>MIGYQIYVRSFRDGNLDGVGDFRGLKNAVSYLKELGIDFVWLMPVFSSISFHGYDVVDFYSFKAEYGSEREFKEMIEAFHDSGIKVVLDLPIHHTGFLHTWFQKALKGDPHYRDYYVWANKETDLDERREWDGEKIWHPLEDGRFYRGLFGPFSPDLNYDNPQVFDEMKRLVLHLLDMGVDGFRFDAAKHMRDTIEQNVRFWKYFLSDLKGIFLAEIWAEARMVDEHGRIFGYMLNFDTSHCIKEAVWKENTRVLIESIERAVI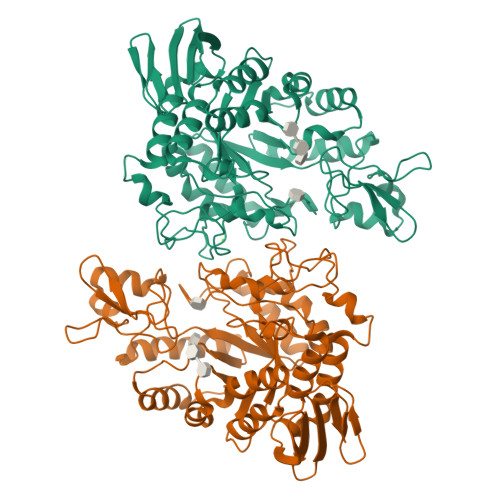AKDYLPVNFTSNHDMSRLASFEGGFSKEKIKLSISILFTLPGVPLVFYGDELGMKGVYQKPNTEVVLDPFPWNESMCVEGQTFWKWPAYNGPFSGISVEYQKRDPDSILSHTLGWTRFRKENQWIDRAKLEFLCKEDKFLVYRLYDDQHSLKVFHNLSGEEVVFEGVKMKPYKTEVV[2x]> SNASQITIQARLISFESNRQQLWKLMADLNTPLINELLCQLGQHPDFEKWQQKGKLPSTVVSQLCQPLKTDPRFAGQPSRLYMSAIHIVDYIYKSWLAIQKRLQQQLDGKTRWLEMLNSDAELVELSGDTLEAIRVKAAEILAIAMPASESDSASPKGKKGKKEKKPSSSSPKRSLSKTLFDAYQETEDIKSRSAISYLLKNGCKLTDKEEDSEKFAKRRRQVEIQIQRLTEKLISRMPKGRDLTNAKWLETLLTATTTVAEDNAQAKRWQDILLTRSSSLPFPLVFE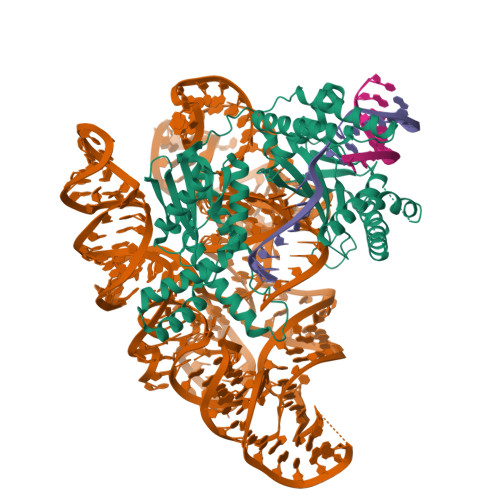TNEDMVWSKNQKGRLCVHFNGLSDLIFEVYCGNRQLHWFQRFLEDQQTKRKSKNQHSSGLFTLRNGHLVWLEGEGKGEPWNLHHLTLYCCVDNRLWTEEGTEIVRQEKADEITKFITNMKKKSDLSDTQQALIQRKQSTLTRINNSFERPSQPLYQGQSHILVGVSLGLEKPATVAVVDAIANKVLAYRSIKQLLGDNYELLNRQRRQQQYLSHERHKAQKNFSPNQFGASELGQHIDRLLAKAIVALARTYKAGSIVLPKLGDMREVVQSEIQAIAEQKFPGYIEGQQKYAKQYRVNVHRWSYGRLIQSIQSKAAQTGIVIEEGKQPIRGSPHDKAKELALSAYNLRLTRRS> ALWQFNGMIKCKIPSSEPLLDFNNYGCYCGLGGS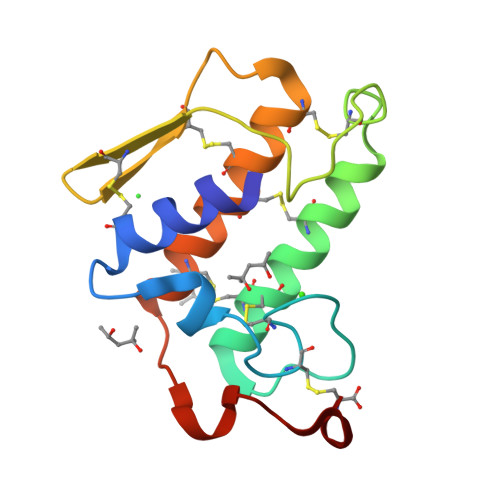GTPVDDLDRCCQTHDNCYMQAMKLDSCKVLVDNPYTNNYSYSCSNNEITCSSENNACEAFICNCDRNAAICFSKVPYNKEHKNLDMKNC>MKKLTIGLIGNPNSGKTTLFNQLTGSRQRVGNWAGVTVERKEGQFSTTDHQVTLVDLPGTYSLTTISSQTSLDEQIACHYILSGDADLLINVVDASNLERNLYLTLQLLELGIPCIVALNMLDIAEKQNIRIEIDALSARLGCPVIPLVSTRGRGIEALKLAIDRYKANENVELVHYAQPLLNEADSLAKVMPS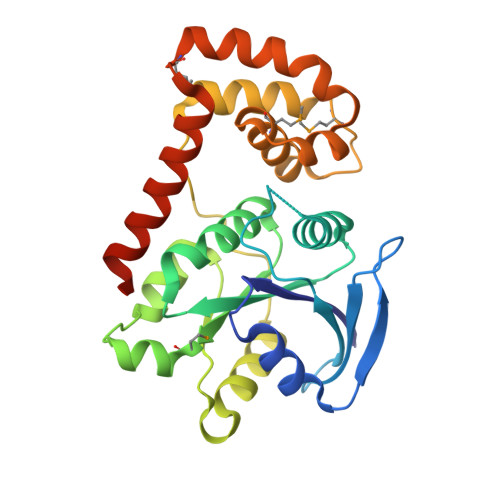DIPLKQRRWLGLQMLEGDIYSRAYAGEASQHLDAALARLRNEMDDPALHIADARYQCIAAICDVVSNTLTAEPSRF[3x]>SAKGDGVTDDTAALTSALNDTPVGQKINGNGKTYKVTSLPDISRFINTRFVYER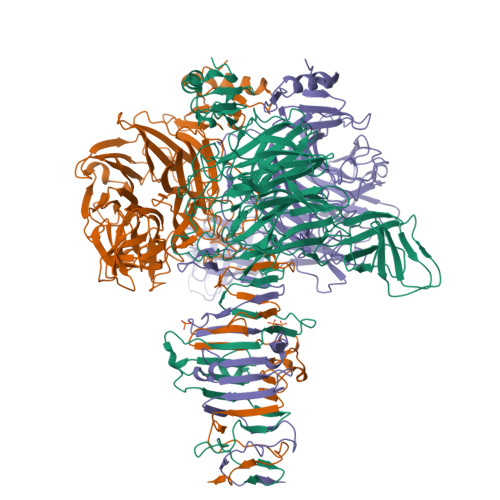IPGQPLYYASEEFVQGELFKITDTPYYNAWPQDKAFVYENVIYAPYMGSDRHGVSRLHVSWVKSGDDGQTWSTPEWLTDLHPDYPTVNYHCMSMGVCRNRLFAMIETRTLAKNALTNCALWDRPMSRSLHLTGGITKAANQRYATIHVPDHGLFVGDFVNFSNSAVTGVSGDMTVATVIDKDNFTVLTPNQQTSDLNNAGKNWHMGTSFHKSPWRKTDLGLIPSVTEVHSFATIDNNGFAMGYHQGDVAPREVGLFYFPDAFNSPSNYVRRQIPSEYEPDASEPCIKYYDGVLYLITRGTRGDRLGSSLHRSRDIGQTWESLRFPHNVHHTTLPFAKVGDDLIMFGSERAENEWEAGAPDDRYKASYPRTFYARLNVNNWNADDIEWVNITDQIYQGGIVNSGVGVGSVVVKDNYIYYMFGGEDHFNPWTYGDNSAKDPFKSDGHPSDLYCYKMKIGPDNRVSRDFRYGAVPNRAVPVFFDTNGVRTVPAPMEFTGDLGLGHVTIRASTSSNIRSEVLMEGEYGFIGKSIPTDNPAGQRIIFCGGEGTSSTTGAQITLYGANNTDSRRIVYNGDEHLFQSADVKPYNDNVTALGGPSNRFTTAYLGSNPIVT[6x]>GAEI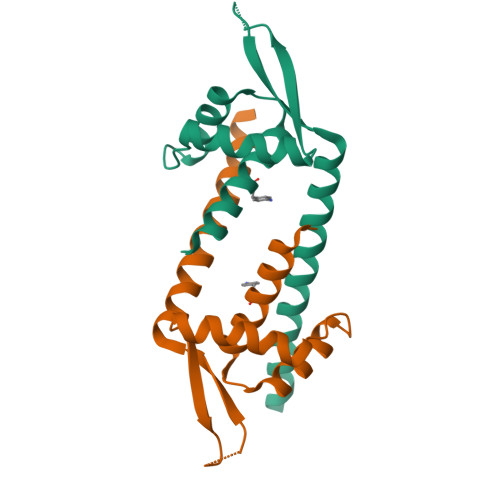PKEMLRAQTNXILLMVLKQGDNYVYGIIKQVKEASNGEMELNEATLYTIFKRLEKDGIISSYWGDESQGGRRKYYRLTEIGHENMRLRHESWSRVDKIIENLEANKKSEAIKSRGGSGGWSHPQFEK[2x]> MMLNIALVILS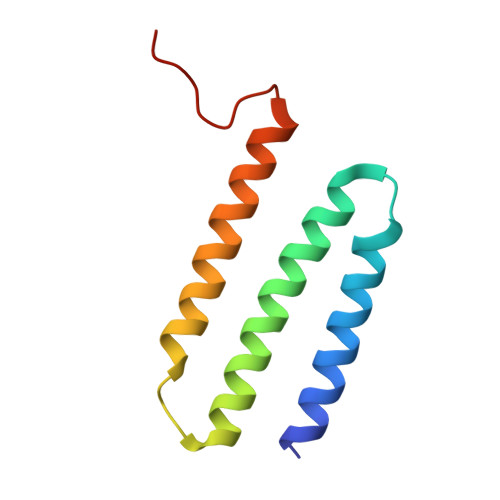LAMVGFLYRVVKGPSTADRIIALDAMGITLAGIVAIVSMLLNTSAFLDVILLIGILAFVGTVAFAKFLEKGVVIERGNDR>[2x]SMGKAPVDPECTAKVGK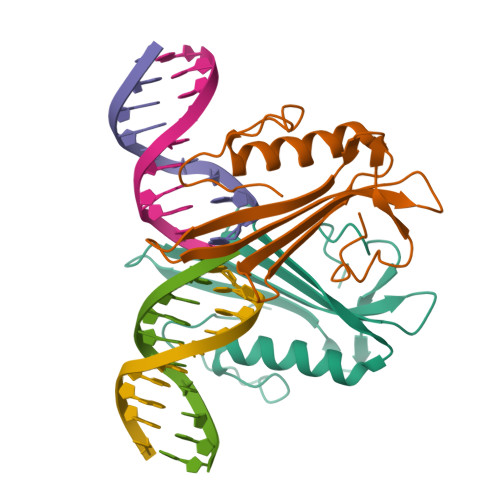AHVYCEGNDVYDVMLNQTNLQFNNNKYYLIQLLEDDAQRNFSVWMRWGRVGKMGQHSLVACSGNLNKAKEIFQKKFLDKTKNNWEDREKFEKVPGKYDMLQMDYATNTQDEEET>MKTITLYLDPASLPALNQLMDFTQNNEDKTHPRIFGLSRFKIPDNIITQYQNIHFVELKDNRPTEALFTILDQYPGNIELNIHLNIAHSVQLIRPILAYRFKHLDRVSIQQLNLYDDGSMEYVDLEKEENKDISAEIKQAEKQLSHYLLTGKIKFDNPTIARYVWQSAFPVKYHFLSTDYFEKAEFLQPLKEYLAENYQKMDWTAYQQLTPEQQAFYLTLVGFNDEVKQSLEVQQAKFIFTGTTTWEGNTDVREYYAQQQLNLLNHFTQAEGDLFIGDHYKIYFKGHPRGGEINDYILNNAKNITNIPANISFEVLMMTGLLPDKVGGVASSLYFSLPKEKISHIIFTSNKQVKSKEDALNNPYVKVMRRLGIIDESQV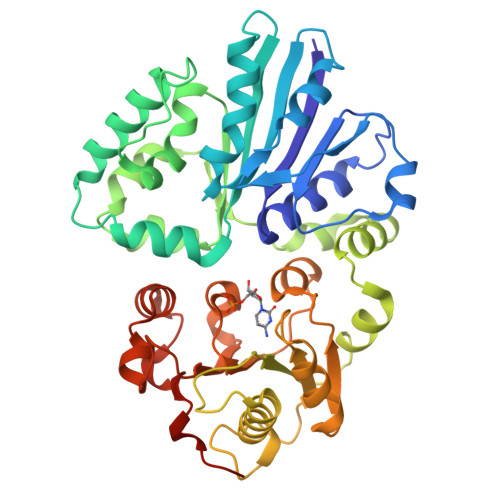IFWDSLKQLGGGLEHHHHHH[2x]> SSNSPSLETDV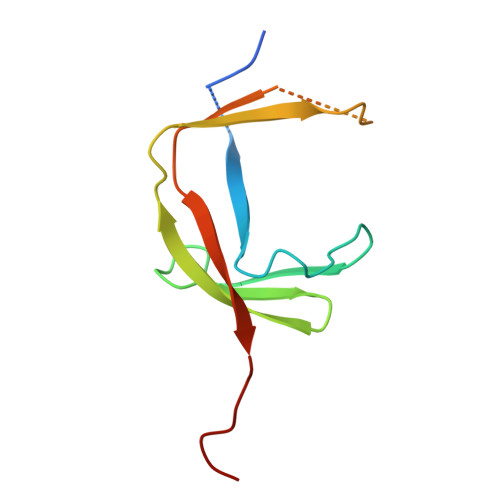DDVENIVFQFQNSSLDFQSSDDFSILGIDQPHPIVRIGGMFFRGTWHQPIGTDIVVPSVNDSELSRDGLVLCKRRLMLEQIRLVPKNPS(4aS,12aS)-3,10,11,12a-tetrahydroxy-6-methyl-1,12-dioxo-1,4,4a,5,12,12a-hexahydrotetracene-2-carboxamide 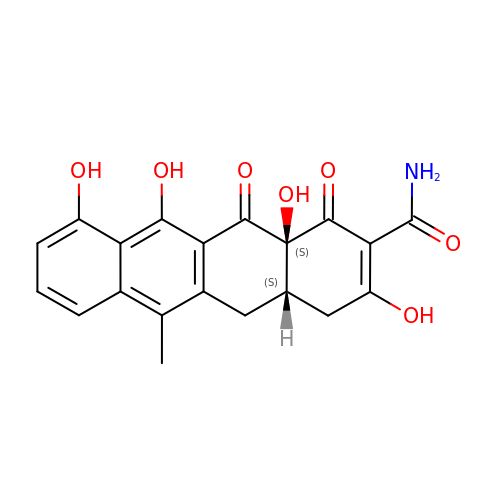| C20 H17 N O7 | UEDQTQIXNDMDID-FHZGZLOMSA-N>[2x]MTSLFTTADHYHTPLGPDGTPHAFFEALRDEAETTPIGWSEAYGGHWVVAGYKEIQAVIQNTKAFSNKGVTFPRFETGEFELMMAGQDDPVHKKYRQLVAKPFSPEATDLFTEQLRQSTNDLIDARI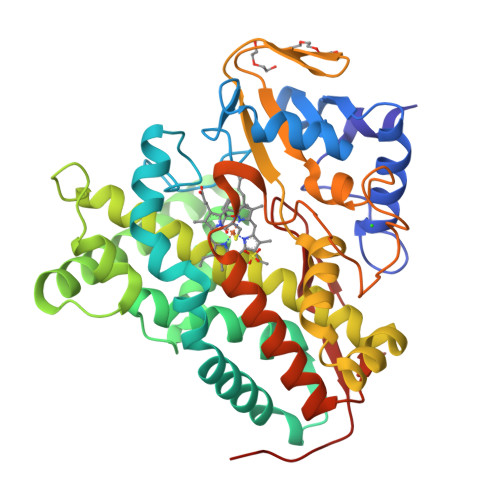ELGEGDAATWLANEIPARLTAILLGLPPEDGDTYRRWVWAITHVENPEEGAEIFAELVAHARTLIAERRTNPGNDIMSRVIMSKIDGESLSEDDLIGFFTILLLGGIDNTARFLSSVFWRLAWDIELRRRLIAHPELIPNAVDELLRFYGPAMVGRLVTQEVTVGDITMKPGQTAMLWFPIASRDRSAFDSPDNIVIERTPNRHLSLGHGIHRCLGAHLIRVEARVAITEFLKRIPEFSLDPNKECEWLMGQVAGMLHVPIIFPKGKRLSE> ILGGREAEAHARPYMASVQLNGAHLCGGVLVAEQWVLSAAHCLEDAADGKVQVLLGAHSLSQPEPSKRLYDVLRAVPHPDSQPDTIDHDLLLLQLSEKATLGPAVRPLPWQRVDRDVAPGTLCDVAGWGIVNHA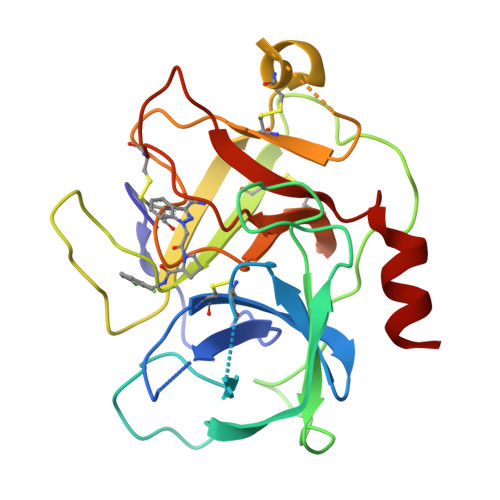GRRPDSLQHVLLPVLDRATCNRRTHHDGAITERLMCAESNRRDSCKGDSGGPLVCGGVLEGVVTSGSRVCGNRKKPGIYTRVASYAAWIDSVLA The recombinant cytokine NGR-TNF, carrying the CNGRC tumor homing peptide, has shown a higher anti-tumor activity than the corresponding wild type cytokine in animal models, thus allowing its use at low, not toxic concentrations. This enhanced efficacy is due to the CNGRC motif that, through the binding to an isoform of the aminopeptidase N (also called CD13), selectively expressed by angiogenic vessels, increases the delivery of the tagged cytokine at the tumor site. Despite the large body of evidence supporting the vascular targeting properties of the NGR-hTNF and its vascular and antitumor effects, a structural and biochemical characterization of the interaction between the recombinant cytokine and its receptors, TNFR and CD13, is still lacking.

Single crystal X-ray diffraction was used to assess whether the CNGRC peptide induces a preferred conformation of the N-terminus of hTNF in the NGR-hTNF molecule. The 2.65 Å crystal structure of NGR-hTNF is substantially identical to that observed in the absence of the N-terminal extension, with a rmsd of 0.81 Å for 373 Cα and 0.95 Å for 2701 total atoms in the trimeric arrangement. The N-terminal region of the mature hTNFα (amino acids 1–8) and the CNGRCG hexapeptide could not be traced due to the lack of a significant continuous electron density in the difference maps. These findings indicate that the N-terminus of the NGR-hTNF molecule does not interact stably with the cytokine, is endowed with very high flexibility and can thus attain many possible orientations. Hence, the crystal structure of NGR-hTNF demonstrates that the targeting peptide in NGR-hTNF does not stabilize a different, specific conformation of the cytokine, and remains available for the interaction with accessory receptors such as CD13. This study superimposed the newly determined structure of NGR-hTNF onto the crystal structure of the lymphotoxin α-TNFR1 complex to model a possible geometry of interaction. In this model, the N-terminal region of NGR-hTNF is positioned between the three TNFR1 molecules, allowing the preceding peptide to extend in the solvent and thus interact with other receptors. These findings suggest that the N-terminal fusion peptide does not hinder the interactions with the TNFR1, and could be available for binding to specific molecular determinants on the cell surface, thus modulating the TNF activity. Taken together, these results demonstrate that the addition of the CNGRC peptide at the N-terminal does not modify the interaction of hTNF with immobilized TNFR1 and TNFR2. These results are consistent with the determined NGR-hTNF structure showing that the N-terminal region is flexible and does not modify the hTNF structure.

>CNGRCGVRSSSRTPSDKPVAHVVANPQAEGQLQWLNRRANALLANGVELRDNQLVVPSEGLYLIYSQVLFKGQGCPSTHVLLTHTISRIAVSYQTKVNLLSAIKSPCQRETPEGAEAKPWYEPIYLGGVFQLEKGDRLSAEINRPDYLDFAESGQVYFGIIAL[3x]5-azanyl-3-[1-[[4-(piperidin-1-ylmethyl)phenyl]methyl]indol-6-yl]-1~{H}-pyrazole-4-carbonitrile | C25 H26 N6 | 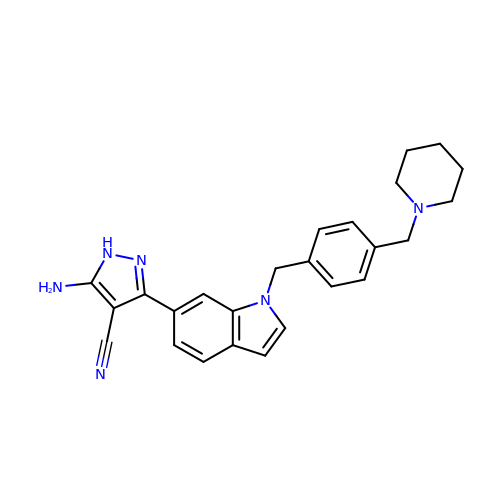OKTJXLZKXVWLTD-UHFFFAOYSA-N> SGRHERDAFDTLFDHAPDKLNVVKKTLITFVNKHLNKLNLEVTELETQFADGVYLVLLMGLLEGYFVPLHSFFLTPDSFEQKVLNVSFAFELMQDGGLEKPKPRPEDIVNCD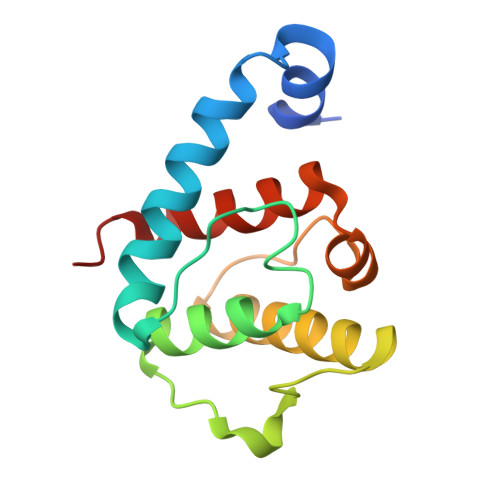LKSTLRVLYNLFTKYRNVE>SMAMFYAHAFGGYDENLHAFPGISSTVANDVRKYSVVSVYNKKYNIVKNKYMWCNSQVNKRYIGALLPMFECNEYLQIGDPIHDLEGNQISIVTYRHKNYYALSGIGYESLDLCLEGVGIHHHVLETGNAVYGKVQHEYSTIKEKAKEMNALKPGPIIDYHVWIGDCVCQVTTVDVHGKEIMRMRFKRGAV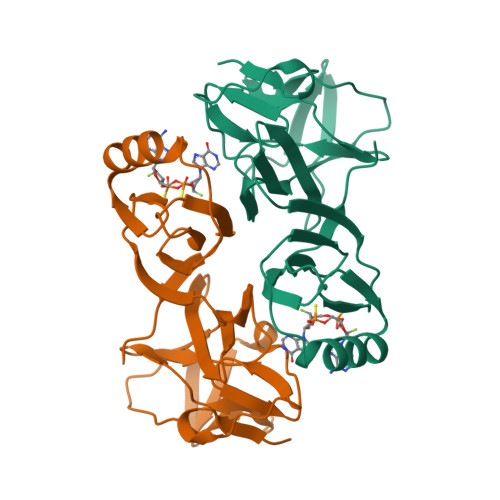LPIPNLV[4x]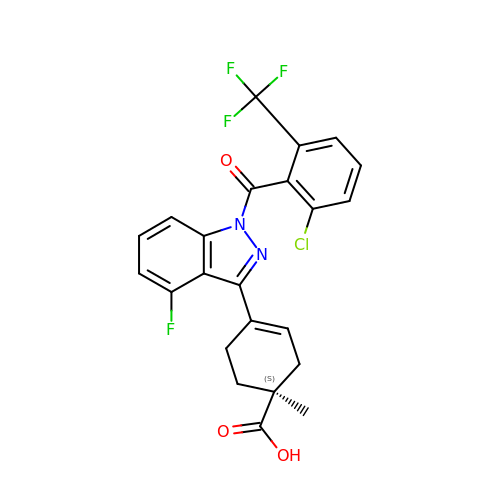(1S)-4-{1-[2-chloro-6-(trifluoromethyl)benzoyl]-4-fluoro-1H-indazol-3-yl}-1-methylcyclohex-3-ene-1-carboxylic acid | C23 H17 Cl F4 N2 O3 | ICXVPFPYYBKMTL-JOCHJYFZSA-N>MSIPVTELRYFADTQPAYRILKPWWDVFTDYISIVMLMIAVFGGTLQVTQDKMICLPCKWVTKDSCNDSFRGWAASSPEPTYPNSTVLPTPDTGPTGIKYDLDRHQYNYVDAVCYENRLHWFAKYFPYLVLLHTLIFLACSNFWFKFPRTSSKLEHFVSILLKCFDSPWTTRALSETVVEESDPKPAFSKMNGSMDKKSSTVSEDVEATVPMLQRTKSRIEQGIVDRSETGVLDKKEGEQAKALFEKVKKFRTHVEEGDIVYRLYMRQTIIKVIKFALIICYTVYYVHNIKFDVDCTVDIESLTGYRTYRCAHPLATLFKILASFYISLVIFYGLICMYTLWWMLRRSLKKYSFESIREESSYSDIPDVKNDFAFMLHLIDQYDPLYSKRFAVFLSEVSENKLRQLNLNNEWTLDKLRQRLTKNAQDKLELHLFMLSGIPDTVFDLVELEVLKLELIPDVTIPPSIAQLTGLKELWLYHTAAKIEAPALAFLRENLRALHIKFTDIKEIPLWIYSLKTLEELHLTGNLSAENNRYIVIDGLRELKRLKVLRLKSNLSKLPQVVTDVGVHLQKLSINNEGTKLIVLNSLKKMVNLTELELIRCDLERIPHSIFSLHNLQEIDLKDNNLKTIEEIISFQHLHRLTCLKLWYNHIAYIPIQIGNLTNLERLYLNRNKIEKIPTQLFYCRKLRYLDLSHNNLTFLPADIGLLQNLQNLAVTANRIEALPPELFQCRKLRALHLGNNVLQSLPSRVGELTNLTQIELRGNRLECLPVELGECPLLKRSGLVVEEDLFSTLPPEVKERLWRADKEQALEVLFQ[4x];>[2x]MSIPVTEFRQFSEQQPAFRVLKPWWDVFTDYLSVAMLMIGVFGCTLQVMQDKIICLPKRVQPAQNHSSVPNVSQAVISTTPLPPPKPSPTNPATVEMKGLKTDLDLQQYSFINQMCYERALHWYAKYFPYLVLIHTLVFMLCSNFWFKFPGSSSKIEHFISILGKCFDSPWTTRALSEVSGEDSEEKDNRKNNMNRSGTIQSGPEGNLVRSQSLKSIPEKFVVDKSAAGALDKKEGEQAKALFEKVKKFRLHVEEGDILYAMYVRQTVLKVIKFLIIIAYNSALVSKVQFTVDCNVDIQDMTGYKNFSCNHTMAHLFSKLSFCYLCFVSIYGLTCLYTLYWLFYRSLREYSFEYVRQETGIDDIPDVKNDFAFMLHMIDQYDPLYSKRFAVFLSEVSENKLKQLNLNNEWTPDKLRQKLQTNAHNRLELPLIMLSGLPDTVFEITELQSLKLEIIKNVMIPATIAQLDNLQELCLHQCSVKIHSAALSFLKENLKVLSVKFDDMRELP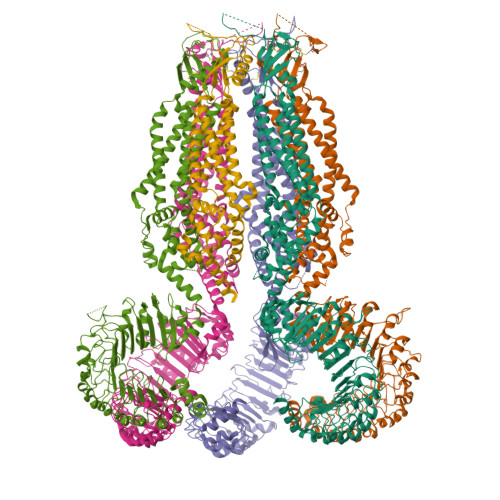PWMYGLRNLEELYLVGSLSHDISKNVTLESLRDLKSLKILSIKSNVSKIPQAVVDVSSHLQKMCVHNDGTKLVMLNNLKKMTNLTELELVHCDLERIPHAVFSLLSLQELDLKENNLKSIEEIVSFQHLRKLTVLKLWYNSIAYIPEHIKKLTSLERLFFSHNKVEVLPSHLFLCNKIRYLDLSYNDIRFIPPEIGVLQSLQYFSITCNKVESLPDELYFCKKLKTLKIGKNSLSVLSPKIGNLLFLSYLDIKGNHFEVLPPELGDCRALKRARLVVEDALFETLPSDVREQMKADALEVLFQ> MAAAAVSGALGRAGWRLLQLRCLPVARCRQALVPRAFHASAVGLRSSDEQKQQPPNSFSQQHSETQGAEKPDPESSHSPPRYTDQGGEEEEDYESEEQLQHRILTAALEFVPAHGWTAEAIAEGAQSLGLSSAAASMFGKDGSELILHFVTQCNTRLTRVLEEEQKLVQLGQAEKRKTDQFLRDAVETRLRMLIPYIEHWPRALSILMLPHNIPSSLSLLTSMVDDMWHYAGDQSTDFNWYTRRAMLAAIYNTTELVMMQDSSPDFEDTWRFLENRVNDAMNMGHTAKQVKSTGEALVQGLMGAAVTLKNLT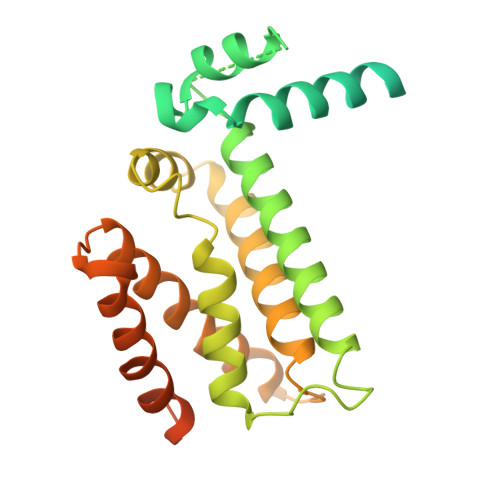GLNQRR> MAKTVEIIEKRFPSGTLASHALVAGDPQSPAVVLLHGAGPGAHAASNWRPIIPDLAENFFVVAPDLIGFGQSEYPETYPGHIMSWVGMRVEQILGLMNHFGIEKSHIVGNSMGGAVTLQLVVEAPERFDKVALMGSVGAPMNARPPELARLLAFYADPRLTPYRELIHSFVYDPENFPGMEEIVKSRFEVANDPEVRRIQEVMFESMKAGMESLVIPPATLGRLPHDVLVFHG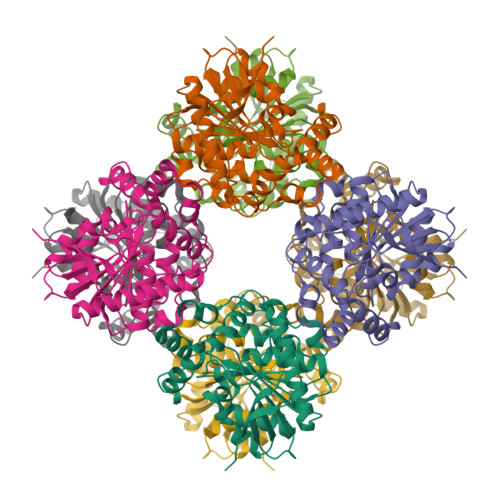RQDRIVPLDTSLYLTKHLKHAELVVLDRCGHWAQLERWDAMGPMLMEHFRAA> ESPLPKPVLDTNGKELNPNSSYRIISIGRGALGGDVY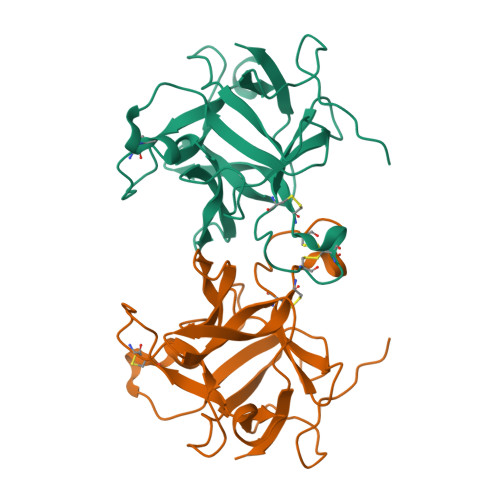LGKSPNSDAPCPDGVFRYNSDVGPSGTPVRFIPLSTNIFEDQLLNIQFNIPTVKLCVSYTIWKVGNLNAYFRTMLLETGGTIGQADNSYFKIVKSSKIGYNLLSCPFTSIICLRCPEDQFCAKVGVVIQNGKRRLALVNENPLDVLFQEV>MGHHHHHHMGGTPHVRGANTRDKIQSVALELFIERGYEKTSMREIAEGLGITKAALYYHFKAKEEILVAISQGLGGPVDELVAWARTQPRTLETKREVLRRYSEALMGAAPLFRIMQESGAALRTLGIGQTLNDRIAAIGELMYQDGASVRSQVRISDALASVHFGAFFLSAIEGDPEEKRKA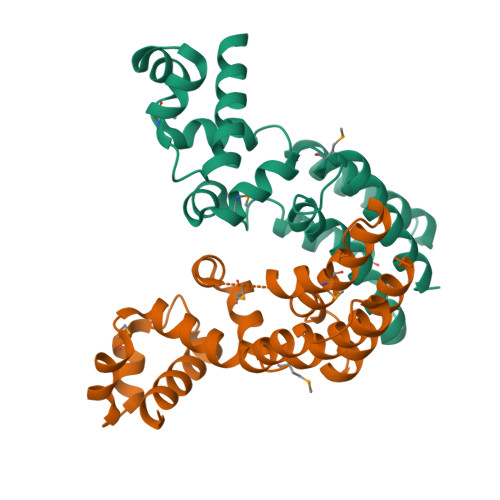LLESALETLDSSAEEDL[4x]> VRNKKVILFDTNHQVSICNQIIDAINSGIDLGDLLEGGLLTLCVEHYYNSDKDKFNTSPIAKYLRDAGYEFDVIKNADATRFLDVIPNEPHYSP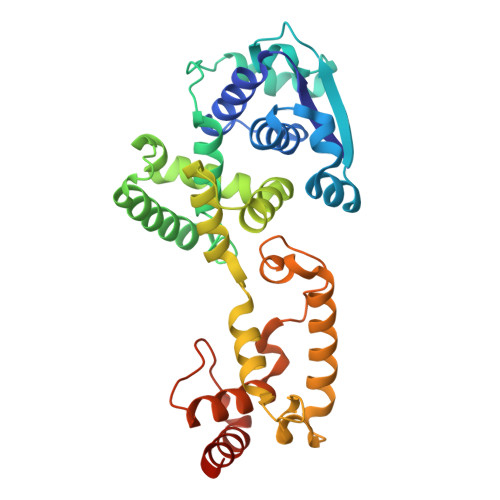LILALKTLESTESQRGRIGLFLSFCSLFLPKLVVGDRASIEKALRQVTVHQEQGIVTYPNHWLTTGHMKVIFGILRSSFILKFVLIHQGVNLVTGHDAYDSIISNSVGQTRFSGLLIVKTVLEFILQKTDSGVTLHPLVRTSKVKNEVASFKQALSNLARHGEYAPFARVLNLSGINNLEHGLYPQLSAIALGVATAHGSTLAGVNVGEQYQQLREAAHDAEVKLQRRHEHQE>[2x]MKQNKLHYTTMIMTQFPDISIQSVESLGEGFRNYAILVNGDWVFRFPKSQQGADELNKEIQLLPLLVGCVKVNIPQYVYIGKRSDGNPFVGYRKVQGQILGEDGMAVFPDDAKDRLALQLAEFMNELSAFPVETAISAGVPVTNLKNKILLLSEAVEDQVFPLLDESLRDYL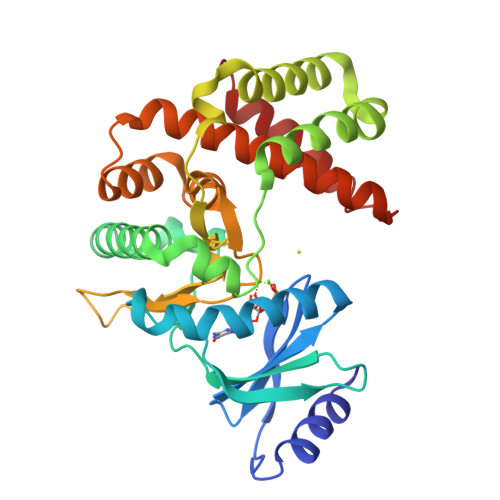TLRFQSYMTHPVYTRYTPRLIHGDLSPDHFLTNLNSRQTPLTGIIDFGDAAISDPDYDYVYLLEDCGELFTRQVMAYRGEVDLDTHIRKVSLFVTFDQVSYLLEGLRARDQDWISEGLELLEEDKANNFGANSA>[2x]SLIELTKMVFQETGKNPV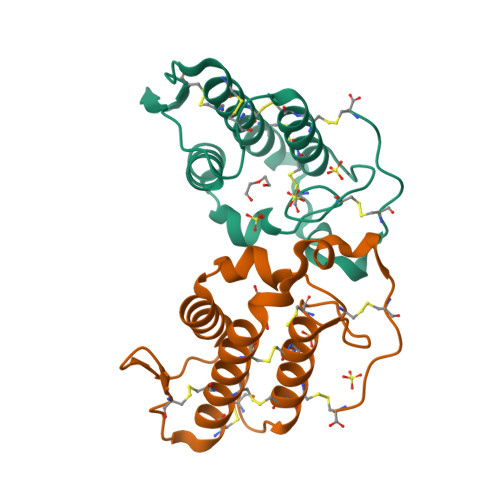TYYTLYGCNCGVGRRGKPKDATDRCCFVHRCCYKKLTGCDPKKDRYSYSWENKAIVCGEKNPCLKELCECDKAVAICLRKNLGTYDKNYRFTMKFLCDKPEKC>[4x]ASMKNCVIVSAVRTAIGSFNGSLASTSAIDLGATVIKA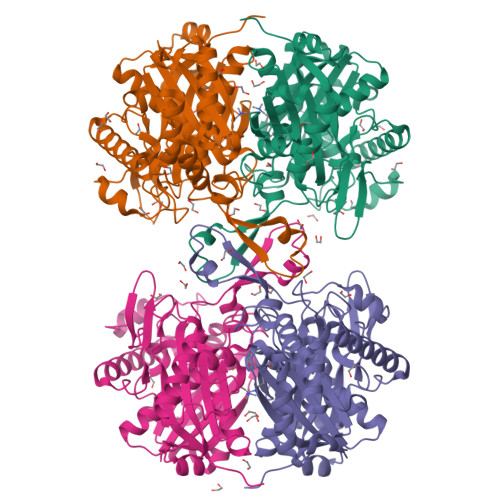AIERAKIDSQHVDEVIMGNVLQAGLGQNPARQALLKSGLAETVCGFTVNKVCGSGLKSVALAAQAIQAGQAQSIVAGGMENMSLAPYLLDAKARSGYRLGDGQVYDVILRDGLMCATHGYHMGITAENVAKEYGITREMQDELALHSQRKAAAAIESGAFTAEIVPVNVVTRKKTFVFSQDEFPKANSTAEALGALRPAFDKAGTVTAGNASGINDGAAALVIMEESAALAAGLTPLARIKSYASGGVPPALMGMGPVPATQKALQLAGLQLADIDLIEANEAFAAQFLAVGKNLGFDSEKVNVNGGAIALGHPIGASGARILVTLLHAMQARDKTLGLATLCIGGGQGIAMVIERL> MSAEKLFTPLKVGAVTAPNRVFMAPLTRLRSIEPGDIPTPLMGEYYRQRASAGLIISEATQISAQAKGYAGAPGLHSPEQIAAWKKITAGVHAEDGRIAVQLWHTGRLSHSSIQPGGQAPVSASALNANTRTSLRDENGNAIRVDTTTPRALELDEIPGIVNDFRQAVANAREAGFDLVELHSAHGYLLHQFLSPSSNQRTDQYGGSVENRARLVLEVVDAVCNEWSADRIGIRVSPIGTFQNVDNGPNEEADALYLIEELAKRGIAYLHMSETDLAGGKPYSEAFRQKVRERFH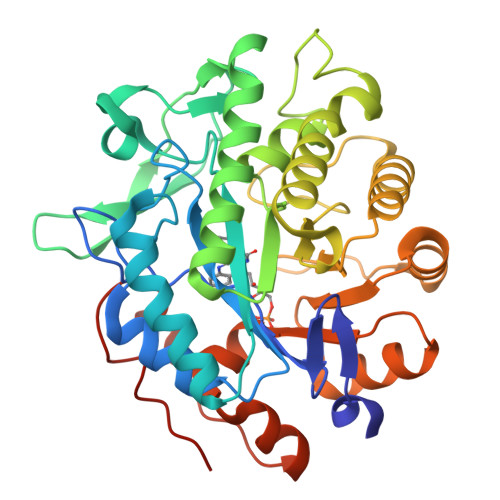GVIIGAGAYTAEKAEDLIGKGLIDAVAFGRDYIANPDLVARLQKKAELNPQRPESFYGGGAEGYTDYPSLHHHHHHHH> GALGVVDEVHAGKEIGLQIYSLSQELYKGDVAANLRKVKDMGYSKLELAGYGKGAIGGVPMMDFKKMAEDAGLKIISSHVNPVDTSISDPFKAMIFKYSKEVTP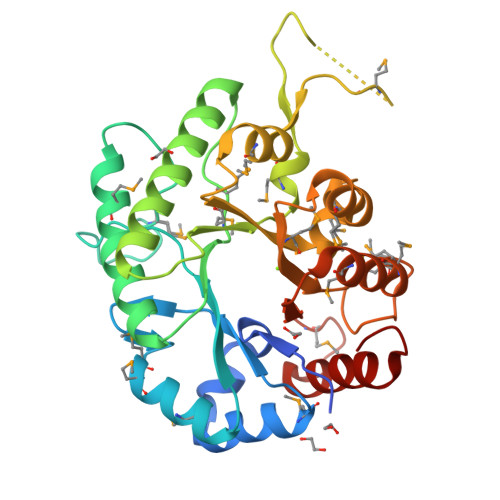KIMEYWKATAADHAKLGCKYLIQPMMPTITTHDEAKLVCDIFNQASDVIKAEGIATGFGYHNHNMEFNRVATKEQQEKVKGNPFAAFMKVGDQIYDLMLKDTDPSKVYFEMDVYWTVMGQNDPVEYMQKHPDRIKVLHIKDRAVFGQSGMMNFEMIFKQMYANGIKDYFVELEQMPDGRTQFAGVKDCADYLIKAPFVK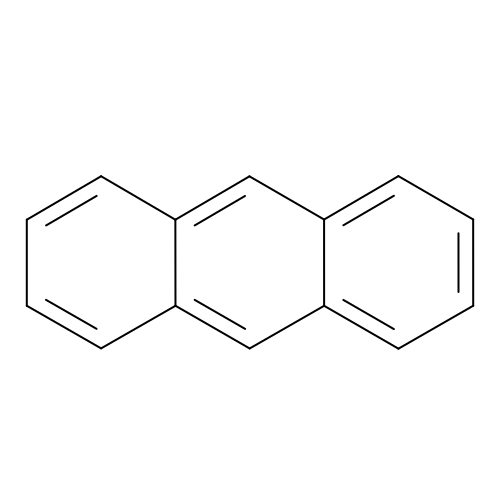ANTHRACENE | C14 H10 | MWPLVEDNUUSJAV-UHFFFAOYSA-N> EQARPADDALAALGAQLFVDPALSRNATQSCATCHDPARAFTDPREGKAGLAVSVGDDGQSHGDRNTPTLGYAALVPAFHRDANGKYKGGQFWDGRADDLKQQAGQPMLNPVEMAMPDRAAVAARLRDDPAYRTGFEALFGKGVLDDPERAFDAAAEALAAYQATGEFSPFDSKYDRVMRGEEKFTPLEEFGYTVFITENCRLCHMQRKQGVAERETFTNFEYHNIGLPVNETAREASGLGADHVDHGLLARPGIEDPAQSGRFKVPSLRNVAVTGPYMHNGVFTDLRTAILFYNKYTSRRPEAKINPETGAPWGEPEVARNLSLAELQSGLMLDDGRVDALVAFLETLT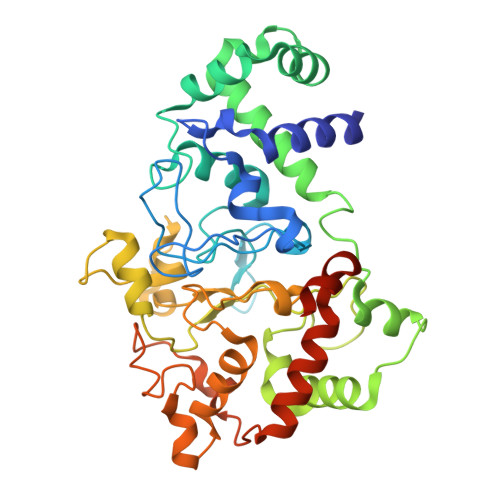DRRYEPLLEESRAAQKDHHHHHH>MNHKVHHHHHHMAKFFTISSSYIKYLKDFDDKVPNSEDPTYNNPKAFIGIVLEIEGHKYLAPLTSPKAWHANVKESSPAFFKLHENGVPDNQLGLINLKFMIPIIEAEVSLLDLDSMPDTPYKRMLYKQLQFIRVNEDKISEKSKLLRNLALQGRMQGTCDFAVLEEKYQHFGKKPEDMEIDDLESR[6x]

In type III TA systems, the toxin is an endoribonuclease (RNase) that cleaves cellular RNAs when free, whereas antitoxin is a noncoding RNA. The toxin also processes its precursor antitoxin RNA into smaller repeats and subsequently assembles with the individual repeats to form an inactive TA complex. The type III TA complexes are unique self-closing RNA–protein assembly, in which the toxin and antitoxin are arranged alternately in a 1:1 ratio. Here, we have chosen to characterize a type III TA system from E. coli ToxIN cluster 1 (strain 680, assembly GCA_001893605.1) in laboratory strains of E. coli such as DH5α.

Crystals were obtained in several conditions; however, crystals obtained under a specific condition in P1 211 space group diffracted to the highest resolution of 2.097 Å at a synchrotron X-ray source. The asymmetric unit contained two hexameric assemblies of TA complexes consisting of six ToxNEc and six ToxIEc repeats. However, the biological assembly comprises of one heterohexameric unit consisting of three ToxNEc and three ToxIEc repeats. The heterohexamer is a cyclic assembly of three proteins bound to three RNA arranged alternately in a head to tail manner. The endoribonuclease toxin ToxNEc is a well-structured protein consisting of five α-helices and seven β-strands. β-strands form the core of the protein that is supported by α-helices on the outside. The core of the antitoxin ToxIEc RNA repeat contains a pseudoknot, which is flanked by single-stranded regions on either side (5′ and 3′ single-stranded regions). ToxIEc forms an H-type pseudoknot consisting of two stems (S1 & S2) and two loops (L1 & L2). There are several base-specific interactions by ToxI at the active site of ToxN involving nucleotides G30, A31, A32, A-3 and U-2. The residues Lys33, Thr52, Ser53, and Lys55 are found at the catalytically active site of ToxN, and the residues Trp57, Phe88, Tyr110 and Gln117 hold the RNA in place for ToxN to cleave the precursor ToxI. The electron density at the active site suggested that the 3′ terminal phosphate of ToxI cyclizes with the 2′-OH of A32 to form a cyclic phosphate, which is an intermediate in RNA cleavage reactions and has also been observed in the previously solved structures of type III TA complexes.1-(4-METHOXYPHENYL)-7-OXO-6-[4-(2-OXOPIPERIDIN-1-YL)PHENYL]-4,5,6,7-TETRAHYDRO-1H-PYRAZOLO[3,4-C]PYRIDINE-3-CARBOXAMIDE | C25 H25 N5 O4 | 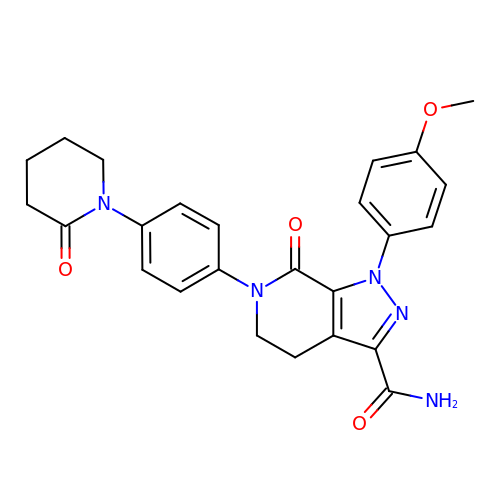QNZCBYKSOIHPEH-UHFFFAOYSA-N4-{3-[3-(methylsulfonyl)phenoxy]phenyl}-8-(trifluoromethyl)quinoline 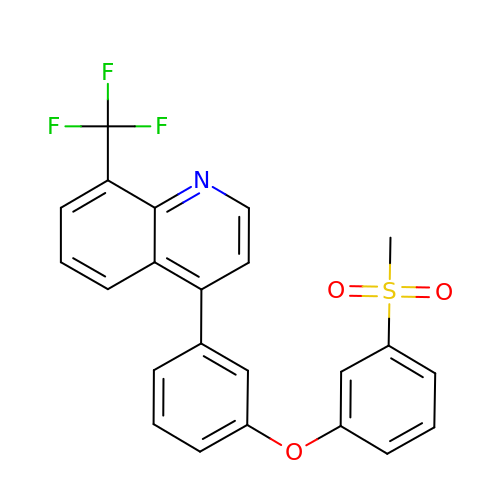| C23 H16 F3 N O3 S | DZEKZLIXNYUATR-UHFFFAOYSA-N> MANVIKTVLTYQLDGSNRDFNIPFEYLARKFVVVTLIG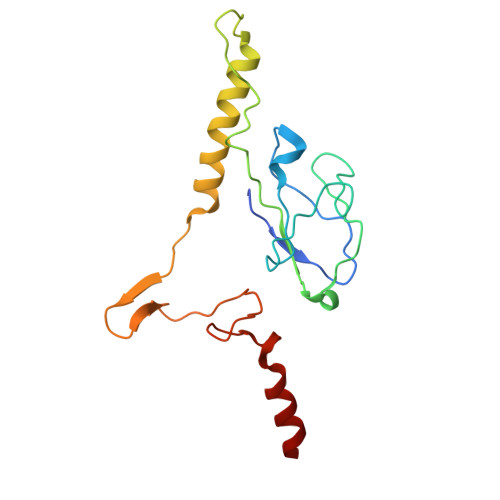VDRKVLTINTDYRFATRTTISLTKAWGPADGYTTIELRRVTSTTDRLVDFTDGSILRAYDLNVAQIQTMHVAEEARDLTTDTIGVNNDGHLDARGRRIVNLANAVDDRDAVPFGQLKTMNQNSWQAR Mitochondrial ATP synthase consists of the soluble F1 and membrane-bound Fo subcomplexes and occurs in dimers that assemble into oligomers to induce the formation of inner-membrane folds, called cristae. Dissociation of ATP synthase dimers into monomers results in the loss of native cristae architecture and impairs mitochondrial function. Here, we report cryo-EM structures of the intact ATP synthase dimer from Trypanosoma brucei in ten different rotational states. Although overall dimer architecture varies among eukaryotes, we find that subunit-g together with subunit-e form an ancestral oligomerization motif, which is shared between the trypanosomal and mammalian lineages.

To describe the conformational space of the T. brucei ATP synthase, we resolved ten distinct rotary substates, which were refined to 3.5–4.3 Å resolution. The three main states (1–3) result from three ~120° rotation steps of the rotor relatively to the static Fo. We identified five (1a–1e), four (2a–2d), and one classes of the respective main states. The rotor positions of the rotational states 1a, 2a, and 3 are related by steps of 117°, 136°, and 107°, respectively. Throughout all the identified substeps of the rotational state 1 (classes 1a to 1e) the rotor turns by ~33°, which corresponds approximately to the advancement by one subunit-c of the c10-ring. While rotating along with the rotor, the F1 headpiece lags behind, advancing by only ~13°. However, due to its large, rigid peripheral stalk, the Polytomella ATP synthase mainly displays rotational substeps, whereas the Trypanosoma F1 also displays a tilting motion of ~8° revealed by rotary states 1a and 1b. Within the four classes of the state 2 the rotor advances by 23° and F1 returns close to its position observed in class 1a, where it is found also in the only observed class of the state 3. In all classes F1 is in a similar conformation, corresponding to the catalytic dwell, observed previously also in the crystal structure of T. brucei F1-ATPase13.

>MRRFGSKFASGLASRCALACPLASAATAPAGASTTSSTSSAQKSFFKTTEMIGYVHSIDGTIATLIPAPGNPGVAYNTIIQIQVSPTTFAAGLVFNLEKDGRIGIILMDNITEVQSGQKVMATGQLLHIPVGAGVLGKVVNPLGHEVPVGLVTRSRRLLDSTLGKVDTGAPNIVSRSPVNYNLLTGFKAVDTMIPIGRGQRELIVGDRQTGKTSIAVSTIINQVRINQQILSKNAVISIYVSIGQRCSNVARIHRLLQSYGALRYTTVMAATAAEPAGLQYLAPYAGVTMGEYFMNRGRHCLCVYDDLSKQAVAYRQISLLLRRPPGREAYPGDVFYLHSRLLERAAMLSPGKGGGSVTALPIVETLSNDVTAYIVTNVISITDGQIYLDTKLFTGGQRPAVNIGLSVSRVGSSAQNAAMKGVAGKLKGILAEYRKLAADSVGGQQVQTIPMIRGARFVALFNQKQPSYFMNAIVSLYACLNGYLDDVKVQYVKFYEYLLVHRDLGIMYGTAKNKFFYMYVQELNYLIRFFTLNSPILHGELEEMLKQHTHLFLQHYQSKMNAIKSEKDVKALKNLLYSCKRAV[3x];>[3x]MLTRFRSAVLRGAVSITGARAASTAPVADHKGRVGHVSQVIGAVVDVHFADGVPPVLTALDVVDKLGRDEPLTLEIVQHLDAHTGRCIAMQTTDLLKLKAKVVSTGGNISVPVGRETLGRIFNVLGDAIDQRGPVGEKLRMPIHAVAPKLADQAAEDAVLTTGIKVIDLILPYCKGGKIGLFGGAGVGKTVIIMELINNVAKGHGGFSVFAGVGERTREGTDLYLEMMQSKVIDLKGESKCVLVYGQMNEPPGARARVAQSALTMAEYFRDVEGQDVLLFIDNIFRFTQANSEVSALLGRIPAAVGYQPTLAEDLGQLQERITSTTKGSITSVQAVYVPADDITDPAPATTFSHLDATTVLDRAVAESGIYPAVNPLECASRIMDPDVISVDHYNVAQDVVQMLTKYRELQDIIAVLGIDELSEEDKLIVDRARKLVKFLSQPFQVAEVFTGMTGHYVQLDDTIDSFSGLLMGTYDQVPEMAFYMVGGINSVLEKAKKMAEEAAELEKMRRARVAQASS;> MSGKLRLYKEKLEGYNRFYSIVKTIKMVTLAKYRAAQGRIRTRDFSLRYTELAFSKPQASRDAVVAAKNALVYIPITTNRGSCGALNSNIVRCIDSVVSSKMVLMPVGKRGIDSFSKLYPDEFRYGIINDMKESMHFGYATFVIENAYEVSKDADRYQVIFNRFVSAGVQRNAVYNIPSYEKWKEDLADAASSDNQKNRYLFANALQNEEEQLIRDFFDFHAALAVLNAVGENELSEQAARLVAVEGQLTNISSLQQRTSSLYNKTRQFGITAALIEILSAMSSLEGNAMKGVRRNKFWEGAVTK;> MFRTFGRRLVSCTLPLLQSAPHDLPEGFEFMEHKVVNKDIHAPHENLETLRLTLTRQDEFLLREEPVKCVTVTGTNGEYGIYPGHAYKIVQLNPSPLTVEYTDGTTKKYFVSGGFAHINNEGSCDVNTVECTLLDDLDLAIAEKELAAQQAALGSAKDDKAKSVVEIRISVIEAVIAALKHH;> MIRRSCALLSSSWRDHGISYLKYLNVCTETLHSTVKESRRAKYERWSKPCYTAQRPDGAGGQETIDKVPIHTKDY;>[3x]MMRRVYSPVFCSVAAARFAATSAAKKYDLFGYEVDTNTAPWIEKIKKCKYYDEAGEVLVNMNVSNCPPDIATYNATLQCIYQSPSKQSTPVDNESKFCAMMDLLEEMQHRNRLKPNEESWTWVMKECVKSGQFRLGYCIQQVMETECKGCPADLVKANEANAQKAKTEGKEHPGHLSQQAGLFDVKVE;>MSAKAAPKTLHQVRNVAYFFAAWLGVQKGYIEKSANDRLWVEHQRKVRQQNVERQQALDSIKLMQQGVRATTPGQLEGVPAELQQLAEAFTK[2x];>[2x]MSSTKCAVACKIMTPLCNAASKVQARSAKKLAALTDAGIQKTISEHNANGTDAAVSSTKRYLAEQRQLFHYRVVRFFDECHYIISGEYFAQYTKVNLIWDLRFLTKLVVLFLIGTVLGRQSIFPPIDPDSPLVEALVTKVNPNY;> MFRRLSSSARAVVAARFYTPPEGLKKLYASDFENSKYPLNIVPSDSVLFAKFLYKAAEEKGNFDNILSDFQKIAAAASKLPIFWERTAVVEKIPEFKQLSEPTFFTLVWMQNNGMLELIQEVAEVYETFVNAKQKKAVAKIFVAPGGEKNVEEARRVAEELHKGLKELADYTLVLKTVVDRTIVKGFAVELAGQYVNKAEGQQKQAGRADEVDYTNLPAPKPQKTVWDDNIETEVLRKYLDGLSQYDMEEAKYGV;>[10x]MMRRLALQSSIRRATPFATPLVASTKALNPMCSAITIREASTVAISVQGLHYVGTGLAAIALAGVGLGIGTIFGNLLVACARQPNLTKMLFNYAILGFALTEAIGLFALMLAFLMLFS;> MFLFFFCDLFWLRLLLCMYYCVWSRLCFIVYFNCLMLIFDFLLFCLFDLYLFVGLCLFLLLWFMLFNLYSLILYYCITYLNLYLLFCIVFLLYIAFLFLFCFLCDFFLFNNLLVGDSFMDVFFIRFLLCFLECFSLLCRCLSTFLRLFCNLLSSHFLLLMFFDFFYFIFVFFFYGVFCYWFILFIFVFCFCLLFYVFLYLLDLFAAILQLFIFCNMILQLIMDFLLFLLFV;> MLRRLGANVSNMARPMNKYAVTVSPRRHLEPMSTWYLASWAMVWYYAFFFWMPMVWTDIMVPSFVYNKLPVIHFLQEKRAEQKLRRVLDETYTEWTEELDQAHVTDAITRSLNI;> MRRVSSPNITIQSVRWISGVSPLLYFPPTTTSTTNREDQINKNTNIAIQMIKRYKGEVPPHYTRKSSATIEQVEKEIDALLGGAEKLRKTSTDDQPMDKLTLMERCLRHALWSYHKEEGRYDFDQIGRWVVYTPEDEVKLAQLKREVEAKEKLAALRKRREEEGLPGGPVPRINWPQEYSSFIDREPVVAKRIRYDTLASTTLERDEKQIESTLQQYRRASQDKRLDDLVDLLERFKPVLAREAIMQRLTIKHLEGQLGVWRYMDWCPEVRDRAELEVDITGWQWWSPLEERRLLPVRLRSVNEVREIMSKTQAKKSAEAAERNPIVTQTSTGDNARDRLLKEVLALQARINQRDEVEPSQTEQKKKAHH;> MQGSWSVLKKNCSNFFPGLLAFAQQTQEAYGIWLRIYNRQQKYGPTDFVEQSETFSPDYHKRFHSQDKNMWVDKELCTEVSQKEVARLMTYKLDMWRMAHCAGALLATGGYAIPFGLFWLANDTWVPSSFNLTGEELRAWREAQDLYRYRSAPSYLTDTKWHFDFHAYPWNETQERAWDDLFEKNDVRRDPKVVRPAAEMYDGFIKFELIRRKSLRHLCRSMNIPTFPMLARLCNGTRVRDYWNLAWCEDYMVITQRLHESMTDEELYDYAWRRYLAPYDKNLNREQLMERVEDYFEFLGPDFVAHGKAPNLVILTNYVLGYYNDPAYLEGDISELDKNDYDHLASWGKDAFLRRLEFENGPLRDQVEAHTQRLLAERAAIAKGDNAAAVEGRHTA;> MVLFSTYRSSRLVSKEFLHGPVMRFRALGEYYFQRAWNGTLNWALPGEYRLYAVMIPFIYFYHRWHNDHTLDRDHVEKAMIMRWGGTLEDVRKLSAKDQLRVRCFTDIEKLYSAYGPKDTYLQPPGDTLPGKDFYRKAGGAQAHH;> MSKQLTFISAGATAAVLQSASAIVSKVAGGRVQTKTAKEAGRHAVVVGPETPIGVHTAVTEVPKSAQDPLFSGVSTVVVRAVLPRAAPDSVQLRDALDVYASAGIDTKEEVRSATEAFKKSAEVAVGKAKAKGVKRIVLVVKQASKHNCINELFKKISTETIESAGLTTEVVGTAAVANQLIVNPESLGVVLLNDVAATEQIELAFAGVVGGVSRVYHTVEGGKISAGHSFKSVALAVAQELRELGLSSEADKVEAAASKNPRAVVSAL;> MRRTFISFSAASAAAAAPVTSTKMQTLHKLLTGEVSFKNKAPVKDCNIVHQFGENWATELSAYAKTLPAEQQKIIVRQIARVKLTRYTVAELAAYCGDGPALLDETARAANIEQGVAFVKAKGVEAFEKYVAEESTNANWKPEEAKKFIEDVKAKAK;> MVYTRWKCDRLPVFQLKLFTQEYPMHAAVGIFTIIFLWKHMSHCSEETERKYGWWAGYPYWRDPIARRNETKYKQMIINNDVDITHPKWTGCSVEQLEELSRVV;> MTKYELKMQYFDEWMIRWRKFQTESDWEIEKGRQWWRRFNMAVSGALFCGLVLYTSGTATLKRQYGLPHFFDIGVDGQAKETMLKTLTSRWRYTPQGYGRVLITGVPTYILFVTLEHYRERRRMQQYLQQNTVFGEQMRRLLSTGKIEEYLPVNIKATLPASQQAIYNY;> MLRRSSAALIRRTPVRHSGGELFVRPKLEEIPPADQCRGFFGPLNDSLKFLRLLDIKWMMNRAVAMRREYLIATPTLFTFIWMFTWKGAVIYFWGDRAPPRRMDWNTEETGRLPLGFKPTPAPL;> MLRKTPLFAMATTRKALVGNGPTFSTGGECMNTCDIQNAFPMNDRGVRSSSPFQEPNTAIYDSYLAWTYFQPMDVHIEKLPAPEAKYYQRHTKKPWDVSSTELTEIQSRKKYFQTLGYLVAFIYLYFLMPKEKSFSGLSGPDGHWIMLPKGRPELF;> MSSGFHFHDVSNDAIKGMPPSEALHKHLENAQLAHRICLAKALKAGEPPVEKCALTWGEVLIRYQAWSEYRPPFQDSVAQAKYKKYWSKKRQEEDDKNPFK;> MLRRLVPRVMMAPMGGATALCTSRGYNMLVFRDPKRRPQLSEEERAKVVVNQAEWPEEFKDFDPDDPYKNSPEIIKGMSSWNLFLWGVECAFIYQFYELVFPKSI;> MTENIEAVMSDFWSNPADHFRPNLKALTLYAERQHYVDRWLHVKERWLAPWYLPWWSPLFQLGTWYSQRSRNLFLVENHLSYRPYKFRRNDEDRNNPY;> MLLGGFVPRRFSQFNRDPCWMFFIFSVGFWLGEYPAMMIKYNARDLVYDPHRYVWSHHDDHH> HPETLVKVKDAEDQLGARVGYIELDLNSGKILESFRPEERFPMMSTFKVLLCGAVLSRIDAGQEQLGRRIHYSQND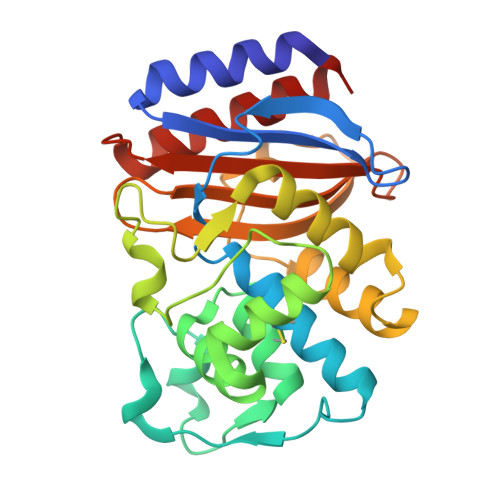LVEYSPVTEKHLTDGMTVRELCSAAITMSDNTAANLLLTTIGGPKELTAFLHNMGDHVTRLDRWEPELNEAIPNDERDTTMPVAMATTLRKLLTGELLTLASRQQLIDWMEADKVAGPLLRSALPAGWFIADKSGAGERGSRGIIAALGPDGKPSRIVVIYTTGSQATMDERDRQIAEIGASLIKHW>[6x]GG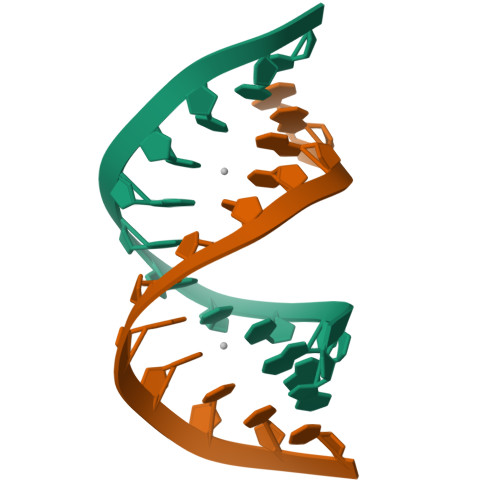GUCCGGUCCC>MSHHHHHHSSGLVPRGSHMLEDLMSKEVSEEAQAHQHGKDYVDPPPAPFFDLGELKLWSFWRAAIAEFIATLLFLYITVATVIGHSKETVVCGSVGLLGIAWAFGGMIFVLVYCTAGISGGHINPAVTFGLFLARKVSLLRALVYMIAQCLGAICGVGLVKAFMKGPYNQFGGGANSVALGYNKGTALGAEIIGTFVLVYTVFSATDPKRSARDSHVPILAPLPIGFAVFMVHLATIPITGTGI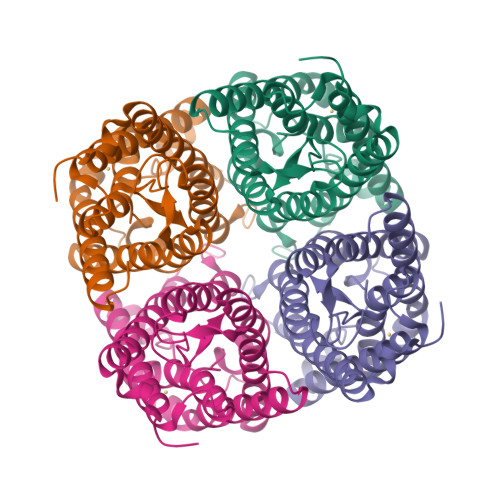NPARSFGAAVIFNSNKVWDDQWIFWVGPFIGAAVAAAYHQYVLRAAAIKALGEFRSNPTN[2x]Many folds, spanning all levels of complexity (fibrous, solenoid, toroid, and globular), clearly originated in this way. β-Propellers offer an attractive model system to study this process. They are toroids formed by sequential supersecondary structure units of typically 40–50 residues, each consisting of four anti-parallel β-strands. The units are arranged radially, with their strands perpendicular to the plane of the toroid, and have a right-handed twist, hence the name ‘propeller’ for the fold and ‘blades’ for the repetitive units. Since none of our single-bladed PkwA constructs were folded, we turned our attention to another highly symmetric β-propeller of the WD40 family, found in the C-terminal part of Npun_R6612 from the multicellular cyanobacterium Nostoc punctiforme PCC 73102 and referred to henceforth as WRAP (WD40-family Recently Amplified Propeller; ACC84870.1). WRAP, which we identified during a systematic bioinformatic survey of β-propellers, was particularly interesting in that its 14 blades are practically identical, having acquired only 10 point mutations over 563 residues (6 of these being Trp → Arg mutations at the same position of blades 1, 3, 6, 10, 12, and 13), as a result of 13 non-synonymous substitutions at the DNA level.

The 4- and 5-bladed constructs assembled into homo-dimers and the 6-bladed construct into homo-tetramers. As we anticipated from their oligomeric states, the 2-bladed and 4-bladed fragments formed 8-bladed propellers and the 3-bladed fragment a 9-bladed propeller. Instead, the packing of the blades within each fragment preserves the geometry of the 7-bladed parent, and the tension due to the mismatch between the number of blades in the assembly versus that in the parent accumulates at the interface between the fragments. The one formed by two 4-bladed fragments absorbs the tension at only two interfaces, leading to an even more pronounced oval shape and a clear two-fold symmetry. This latter construct, unlike all others, also shows considerable interface variability between the propellers in the asymmetric unit of the crystal, resulting from the two halves being shifted to different extent in the plane of the interface, further highlighting the inherent structural tension.

>[6x]GAMGSSSVWGVAFSPDGQTIASASDDKTVKLWNRNGQLLQTLTGHSSSVWGVAFSPDGQTIASASDDKTVKLWNRNGQLLQTLTGHSSSVWGVAFSPDGQTIASASDDKTVKLWNRNGQLLQTLTGHSSSVWGVAFSPDGQTIASASDDKTVKLWNRNGQLLQTLTGH> GLASANVDFAFSLYKQLVLKAPDKNVIFSPLSISTALAFLSLGAHNTTLTEILKGLKFNLTETSEAEIHQSFQHLLRTLNQSSDELQLSMGNAMFVKEQLSLLDRFTEDAKRLYGSEAFATDFQDSAAAKKLINDYVKNGTRGKITDLIKDLDSQTMMVLVNYIFFKAKWEMPFDPQDTHQSRFYLSKKKWVMVPMMSLHHLTIPYFRDEELSCTVVELKYTGNASALFILPDQDKMEEVEAMLLPETLKRWRDSLEFREIGELYLPKFSISRDYNLNDILLQLGIEEAFTSKADLSGITGARNLAVSQVVHKAVLDVFEEGT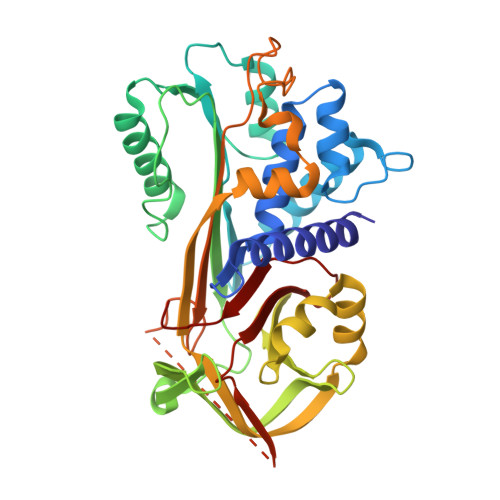EASAATAVKITLLSALVETRTIVRFNRPFLMIIVPTDTQNIFFMSKVTNPKQ>ETFTVKMGADSGLLQFEPANVTVHPGDTVK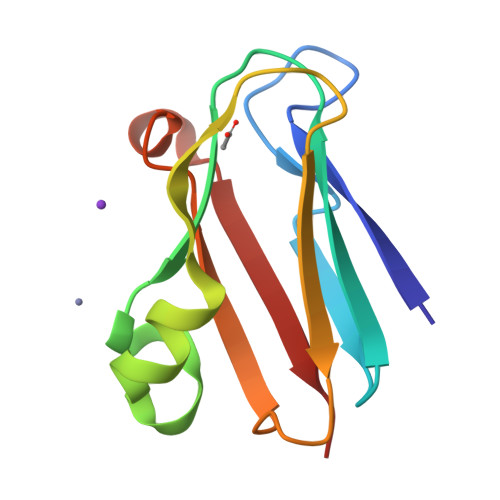WVNNKLPPHNILFDDKQVPGASKELADKLSHSQLMFSPGESYEITFSSDFPAGTYTYYCAPHRGAGMVGKITVEG[3x]>MAGAKRLELGEALALGSGWRHVCHALLYAPDPGMLFGRIPLRYAILMQMRFDGRLGFPGGFVDTQDRSLEDGLNRELREELGEAAAAFRVERTDYRSSHLTEGPHRVVAHFYAKRLTLEELLAVEAGATRAKDHGLEVLGLVRVPLYTLRDGVGGLPTFLENSFIGSAREQLLEALQDLGLLQSGSISGLKIPAHH[2x];>GHMNSFVGLRVVAKWSSNGYFYSGKITRDVGAGKYKLLFDDGYECDVLGKDILLCDPIPLDTEVTALSEDEYFSAGVVKGHRKESGELYYSIEKEGQRKWYKRMAVILSLEQGNRL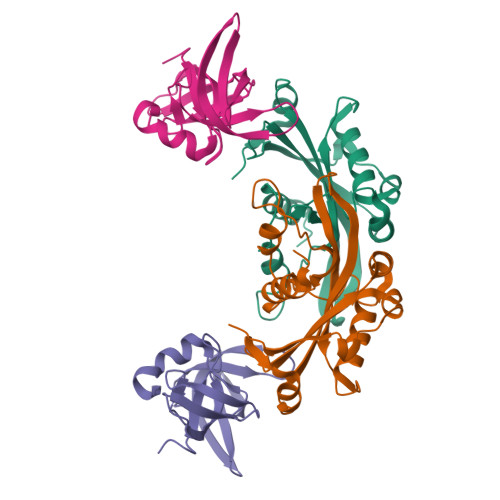REQYGLG[2x]>[2x]MKHQHQHQHQHQHQQPLQEEEQAHATSLPPRASSPPQILPQLSPEQLGMIEKLVAAQQQCNRRSFSDRLRVTPWPMAPDPHSREARQQRFAHFTELAIVSVQEIVDFAKQLPGFLQLSREDQIALLKTSAIEVMLLETSRRYNPGSESITFLKDFSYNREDFAKAGLQVEFINPIFEFSRAMNELQLNDAEFALLIAISIFSADRPNVQDQLQVERLQHTYVEA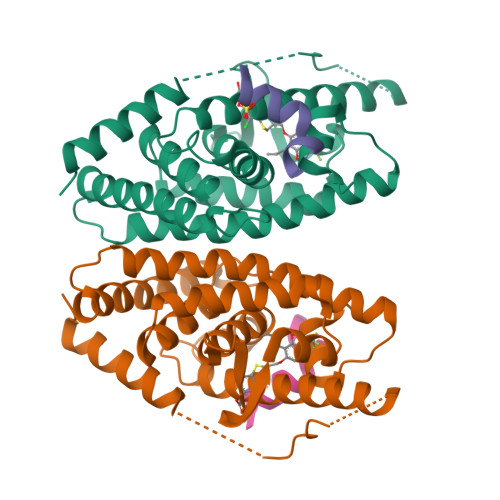LHAYVSIHHPHDRLMFPRMLMKLVSLRTLSSVHSEQVFALRLQDKKLPPLLSEIWDVHE;>[2x]CPSSHSSLTERHKILHRLLQEGSPS> MASRSVIRSIIKSSRLEEDRKRYLMTLLDDIKGANDLAKFHQM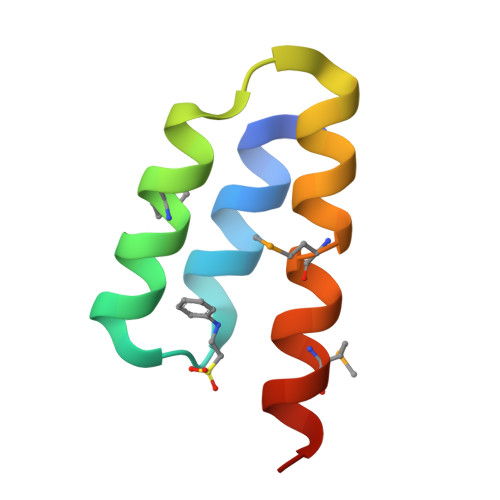LVKIIMKHHHHHH> GAMDPMATGDLKRSLRNLEQVLRLLNYPEEVDCVGLIKGDPAASLP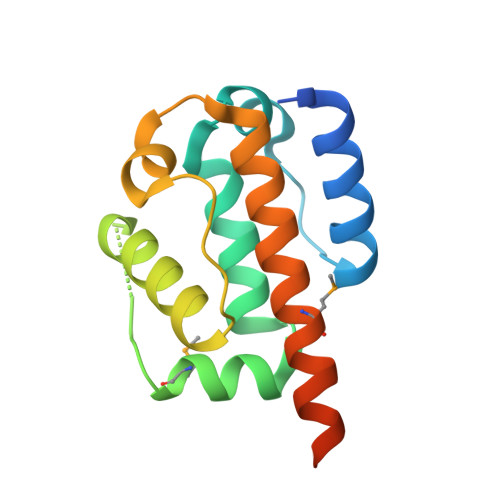IISYSFTSYSPYVTELIMESNVELIAKNDLRFIDAVYKLLRDQFNYKPILTKKQFIQCGFAEWKIQIVCDILNCVMKKHKELSSLQKIPSQQRKKISSG>MSLDKLLERFLNYVSLDTQSKAGVRQVPSTEGQWKLLHLLKEQLEEMGLINVTLSEKGTLMATLPANVPGDIPAIGFISHVDTSPDCSGKNVNPQIVENYRGGDIALGIGDEVLSPVMFPVLHQLLGQTLITTDGKTLLGADDKAGIAEIMTALAVLQQKKIPHGDIRVAFTPDEEVGKGAKHFDVDAFDARWAYTVDGGGVGELEFENFNAASVNIKIVGNNVHPGTAKGVMVNALSLAARIHAEVPADESPEMTEGYEG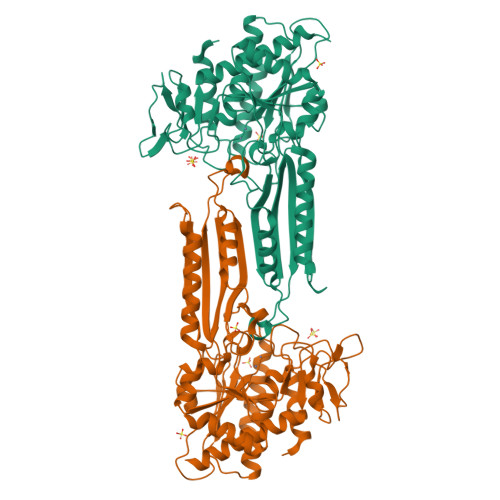FYHLASMKGTVERADMHYIIRDFDRKQFEARKRKMMEIAKKVGKGLHPDCYIELVIEDSYYNMREKVVEHPHILDIAQQAMRDCDIEPELKPIRGGTDGAQLSFMGLPCPNLFTGGYNYHGKHEFVTLEGMEKAVQVIVRIAELTAQRKEGGSHHHHHH[2x]> MAEQVALSRTQVCGILREELFQGDAFHQSDTHIFIIMGASGDLAKKKIYPTIWWLFRDGLLPENTFIVGYARSRLTVADIRKQSEPFFKATPEEKLKLEDFFARNSYVAGQYDDAASYQRLNSHMNALHL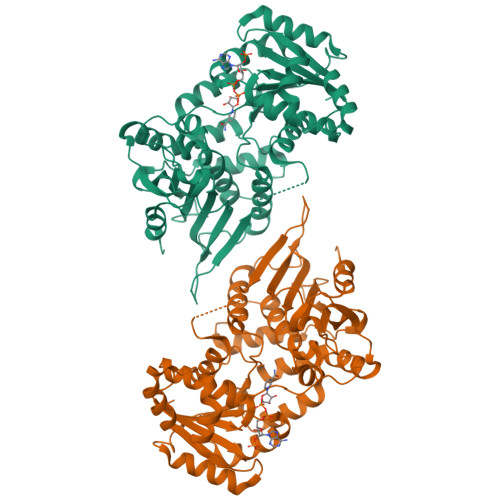GSQANRLFYLALPPTVYEAVTKNIHESCMSQIGWNRIIVEKPFGRDLQSSDRLSNHISSLFREDQIYRIDHYLGKEMVQNLMVLRFANRIFGPIWNRDNIACVILTFKEPFGTEGRGGYFDEFGIIRDVMQNHLLQMLCLVAMEKPASTNSDDVRDEKVKVLKCISEVQANNVVLGQYVGNPDGEGEATKGYLDDPTVPRGSTTATFAAVVLYVENERWDGVPFILRCGKALNERKAEVRLQFHDVAGDIFHQQCKRNELVIRVQPNEAVYTKMMTKKPGMFFNPEESELDLTYGNRYKNVKLPDAYERLILDVFCGSQMHFVRSDELREAWRIFTPLLHQIELEKPKPIPYIYGSRGPTEADELMKRVGFQYEGTYKAVNPHKL>GSHMRQPIALISVHGDPAADVGHESAGGQNIYVRQLGEALAAAGWHVDMFTRKTDPNDPDVIEHSPHCRTIRLQAGPLTYIPREKLFETLPKFVEAFKAYHAKYGYPLIHTNYWLSGWVGWQLRQQFNFQWLHTYHSLGVVKYQVASEQAQRDETRLMVEKAILENADCVIVTSPQEEAYLRRWVSKAGQTRLIPCGTNWEAIALQMGQLYRQLFAASL[4x]

SPS catalyzes sucrose-6-phosphate (S6P) synthesis by using UDP-glucose and fructose-6-phosphate. All SPSs identified so far belong to the GT-B type glucosyltransferase family and contain two Rossmann-type folds. The N-terminal fold is called the A-domain and the C-terminal fold is called the B-domain. Thermosynechococcus elongatus SPS is a kind of sucrose-phosphate synthase (EC 2.4.1.14).

In order to study the function of TeSPS A- and B- domains, we generated three truncated proteins. In the second one, the last α6 helix was switched to the C-terminus of the first one, with this truncated protein having the entire A-domain. All three truncated proteins were easily purified from E.coli. However, only the second protein (residues 27–220 and 406–426) could be crystallized and resolved to 1.92 Å with structural statistics provided in Table 1. The A-domain could be merged perfectly with the A-domain of the full-length enzyme with an RMSD of 1.3 Å. Unlike the first truncated protein, this one has the α6 helix at the C-terminus, implying that the α6 helix in this position is important for domain folding. However, in the second truncated protein, electron densities of two loops (loop 1, residues 37-52, and loop 2, residues 160–173) were relatively poor and thus their structures could not be solved. In the full-length enzyme, loop 1 is key to binding UDP and loop 2 is close to S6P. In apo-TeSPS, these loops are likely flexible and appear to be important for enzyme-substrate binding. In the absence of UDP binding, loop 1 was crystallographically invisible in the A-domain structure. MD analysis of the A-domain shows that RMSD values of loop 1 and loop 2 are higher than those in the full-length enzyme.XIAP (X-linked inhibitor of apoptosis) directly inhibits the upstream caspase-9 and the downstream caspase-3 and caspase-7, and therefore controls critical apoptotic checkpoints. The XIAP protein consists of several domains, including three zinc-containing BIR (baculovirus IAP repeat) domains (BIR1, BIR2 and BIR3) and a C-terminal RING domain. The linker region blocks the active sites of these caspases, while the N-terminal regions of the partially processed caspase-3 and caspase-7 bind the BIR2 domain in a peptide-binding groove that accommodates the four N-­terminal residues. As has been reported previously for other BIR domains, the overall architecture of the BIR2 domain is a three-stranded antiparallel β-sheet surrounded by five α-helices, with a structurally important zinc residue coordinated by Cys200, Cys203, His220 and Cys227.

Therefore, the structures of XIAP BIR2 with five different peptides soaked in and bound to the Smac binding groove were also solved: ATAA, AVPI, SVPI, AIAV and AMRV. Next, AIAV binds identically to SVPI, but with an intermediate position observed for Gln197, which does not have to move as much to accommodate the valine as it does for the isoleucine. The Gln197 can move away, resulting in a pocket that allows longer moieties in this pocket, as was shown in the P4 Ala→Val→Ile series. We have shown in a series of peptide-bound structures that the protein is somewhat flexible and can adjust the conformation of the side chains in the binding groove to accommodate differences in the peptide.

>[2x]GTIYPRNPAMYSEEARLKSFQNWPDYAHLTPRELASAGLYYTGIGDQVQCFACGGKLKNWEPGDRAWSEHRRHFPNCFFVLGRNLN;> AIAV> MQSPHAKYLRECLSLAEKSPPRPTNFRVGAILVSRKEGDYKTEDDRIVSTGYTMELAGNTHAEQCCLSNYAAVHSVPEDRVWEVLPSEPDRKLVMYVTMEPCGKRLSGNLPCVQRIIRTRQGDRKGIQKIYFGVKEPGTFVGGSEGCQMLTA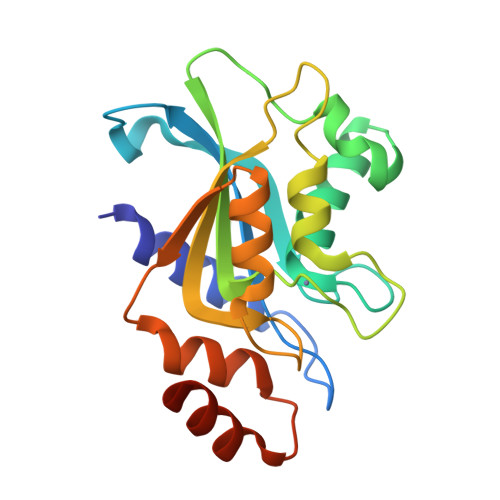AGIDWQVVNGLEREILEVAVAGHENREEEVKAALDTLEHHHHHH> GAMTKPRFTTGLVYDTLMLKHQCTCGSSSSHPEHAGRIQSIWSRLQETGLRGKCECIRGRKATLEELQTVHSEAHTLLYGTNPLNRQKLDSKKLLGSLASVFVRLPCGGVGVDSDTIWNEVHSAGAARLAVGCVVELVFKVATGELKNGFAVVRPPGHHAEESTPMGFCYFNSVAVAAKLLQQRLSVSKILIVDWDVHHGNGTQQAFYSDPSVLYMSLHRYD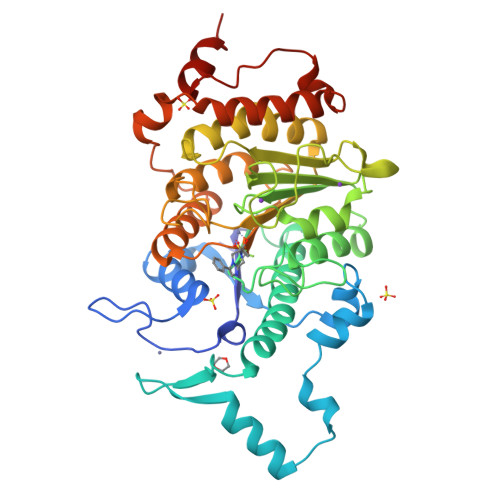DGNFFPGSGAPDEVGTGPGVGFNVNMAFTGGLDPPMGDAEYLAAFRTVVMPIASEFAPDVVLVSSGFDAVEGHPTPLGGYNLSARCFGYLTKQLMGLAGGRIVLALEGGHDLTAICDASEACVSALLGNELDPLPEKVLQQRPNANAVRSMEKVMEIHSKYWRCLQRTTSTAGRSLIEAQTCENEEAETVT> IFPKQYPIINFTTAGATVQSYTNFIRAVRGRLTTGADVRHEIPVLPNRVGLPINQRFILVELSNHAELSVTLALDVTNAYVVGYRAGNSAYFFHPDNQEDAEAITHLFTDVQNRYTFAFGGNYDRLEQLAGNLRENIELGNGPLEEAISALYYYSTGGTQLPTLARSFIICIQMISEAARFQYIEGEMRTRIRYNRRSAPDPSVITLENSWGRLSTAIQESNQGAFASPIQLQRRNGSKFSVYDVSILIPIIALMVYRCAPPPSSQF;> ADV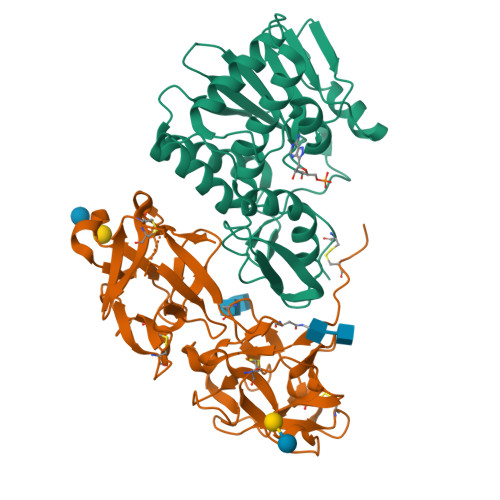CMDPEPIVRIVGRNGLCVDVRDGRFHNGNAIQLWPCKSNTDANQLWTLKRDNTIRSNGKCLTTYGYSPGVYVMIYDCNTAATDATRWQIWDNGTIINPRSSLVLAATSGNSGTTLTVQTNIYAVSQGWLPTNNTQPFVTTIVGLYGLCLQANSGQVWIEDCSSEKAEQQWALYADGSIRPQQNRDNCLTSDSNIRETVVKILSCGPASSGQRWMFKNDGTILNLYSGLVLDVRASDPSLKQIILYPLHGDPNQIWLPLF>[5x]GAMGQTSTRWTPTTEQIKILKELYYNNAI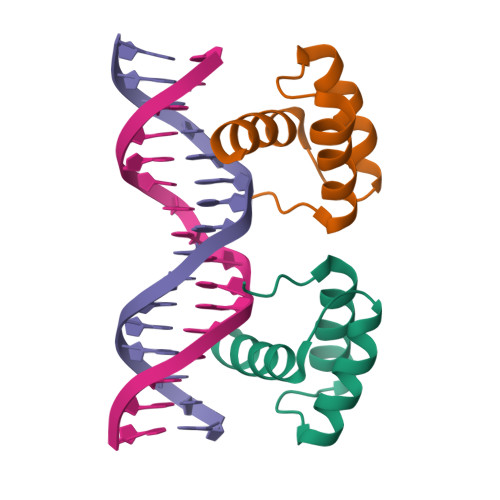RSPTADQIQKITARLRQFGKIEGKNVFYWFQNHKARERQKKRFNGGS>[2x]HH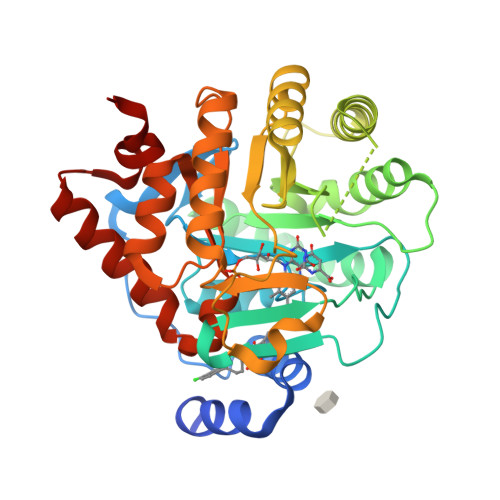HHHHATGDDHFYAEYLMPGLQRLLDPESAHRLAVRVTSLGLLPRATFQDSDMLEVKVLGHKFRNPVGIAAGFDKNGEAVDGLYKLGFGFVEVGSVTPQPQEGNPRPRVFRLPEDQAVINRYGFNSHGLSVVEHRLRARQQKQAQLTADGLPLGINLGKNKTSEDAAADYAEGVRTLGPLADYLVVNVSSPNTAGLRSLQGKTELRHLLSKVLQERDALKGTRKPAVLVKIAPDLTAQDKEDIASVARELGIDGLIVTNTTVSRPVGLQGALRSETGGLSGKPLRDLSTQTIREMYALTQGRIPIIGVGGVSSGQDALEKIQAGASLVQLYTALIFLGPPVVVRVKRELEALLKERGFTTVTDAIGADHRR>GGGGT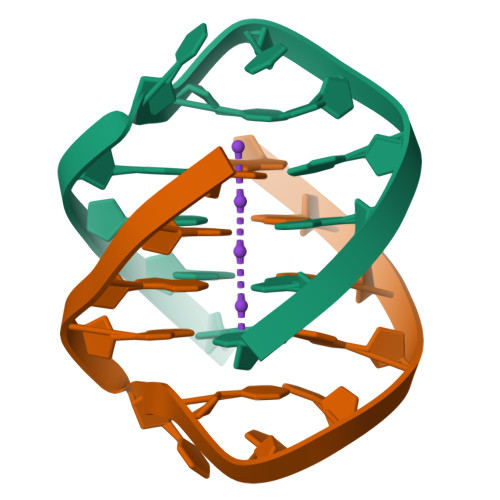TTTGGGG[12x]>[2x]GAAUUGCGGGAAAGGGGUCAACAGCCGUUCAGUACCAAGUCUCAGGGGAAACUUUG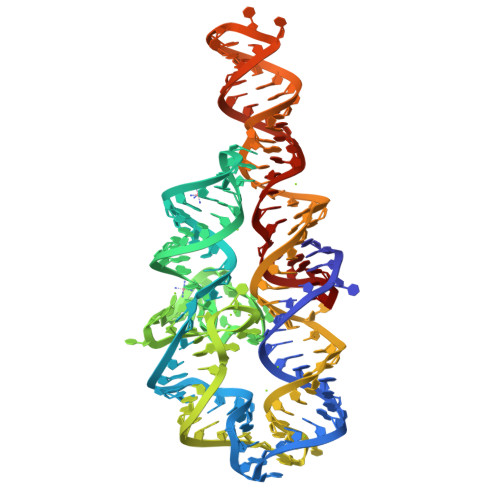AGAUGGCCUUGCAAAGGGUAUGGUAAUAAGCUGACGGACAUGGUCCUAACCACGCAGCCAAGUCCUAAGUCAACAGAUCUUCUGUUGAUAUGGAUGCAGUUC OXIRANPSEUDOGLUCOSE | C7 H12 O5 | 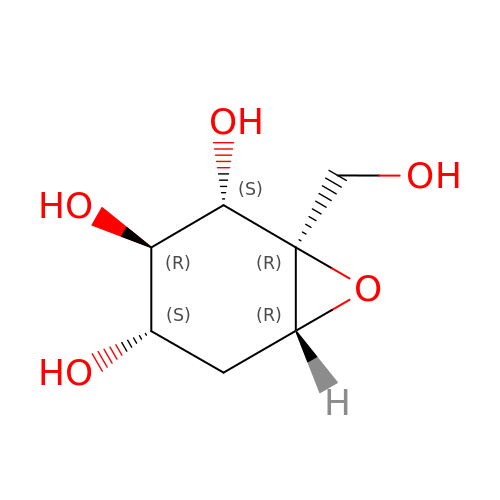BDIDRHMZXLEMIZ-CXNFULCWSA-N> GAQVSTQKTGAHETGLNASGNSII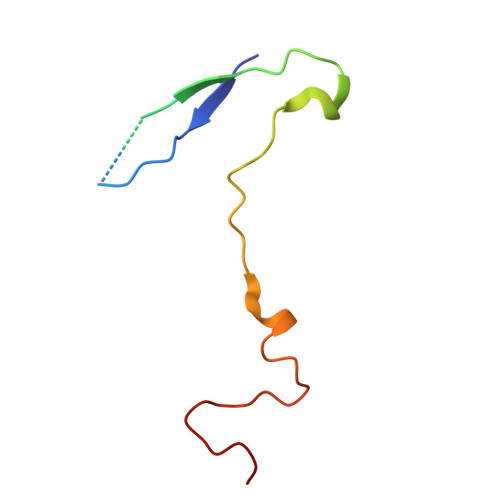HYTNINYYKDAASNSANRQDFTQDPSKFTEPVKDIMIKSLPALN> MSLNNYTIKDITRASGGFAMLAVDQREAMRLMFAAAGAKTPVADSVLTDFKVNAAKILSPYASAVLLDQQFCYRQAVEQNAVAKSCAMIVAADDFIPGNGIPVDNVVLDKKINAQAVKRDG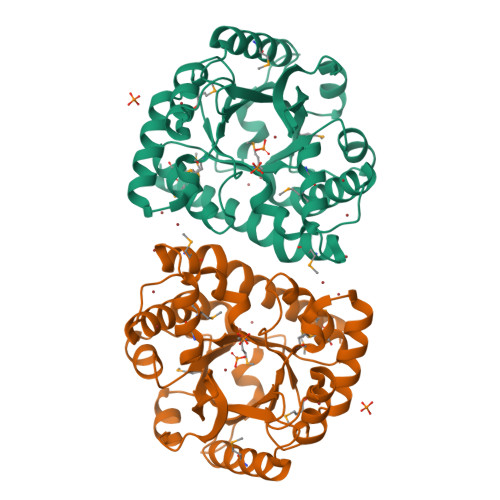AKALKLLVLWRSDEDAQQRLNMVKEFNELCHSNGLLSIIEPVVRPPRCGDKFDREQAIIDAAKELGDSGADLYKVEMPLYGKGARSDLLTASQRLNGHINMPWVILSSGVDEKLFPRAVRVAMEAGASGFLAGRAVWSSVIGLPDTELMLRDVSAPKLQRLGEIVDEMMGKRREGGSHHHHHH> WQPPWYCKEP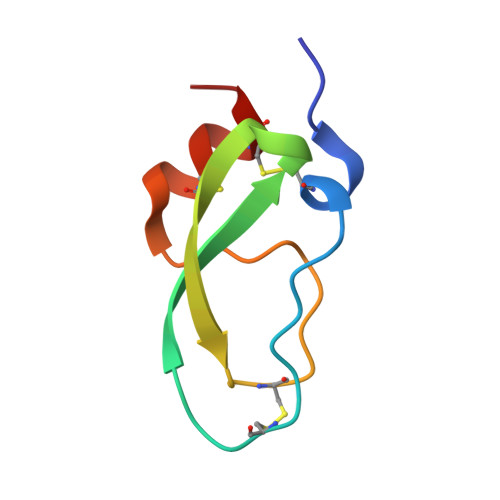VRIGSCKKQFSSFYFKWTAKKCLPFLFSGCGGNANRFQTIGECRKKCLGK> SPILGYWKIKGLVQPTRLLLEYLEEKYEEHLYERDEGDKWRNKKFELGLEFPNLPYYIDGDVKLTQSMAIIRYIADKHNMLGGCPKERAEISMLEGAVLDIRYGVSRIAYSKDFETLKVDFLSKLPEMLKMFEDRLCHKTYLNGDHVTHPDFMLYDALDVVLYMDPMCLDAFPKLVCFKKRIEAIPQIDKYLKSSKYIAWPLQGWQATFGGGDHPPKSDLVPRGS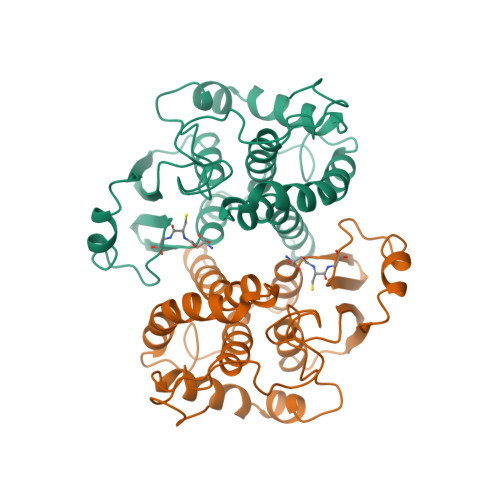MELDKWA(2M)-4'-(hydroxymethyl)-2-(1H-tetrazol-5-yl)[1,1'-biphenyl]-3-ol | C14 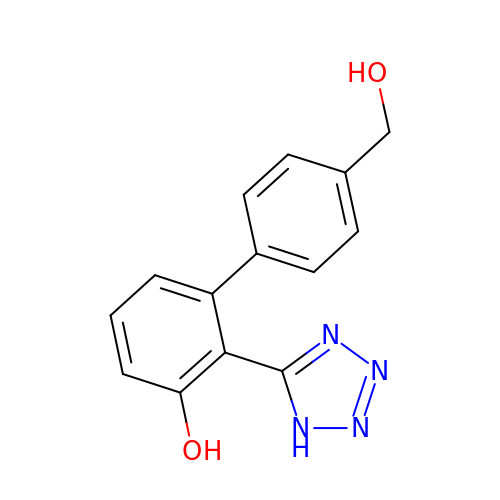H12 N4 O2 | MHFBCDLPGNNTMV-UHFFFAOYSA-N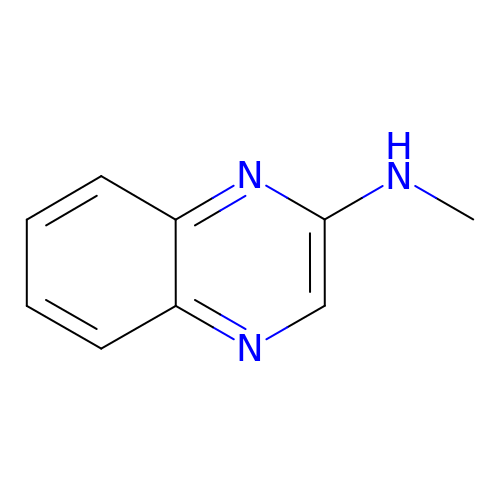N-methylquinoxalin-2-amine | C9 H9 N3 | ILHBRNLXKVETML-UHFFFAOYSA-N> RKKIHQWYYRADDLEHKTALLVHLLKQPEATRSIVFVRKRERVHELANWLREAGINNCYLEGEMVQGKRNEAIKRLTEGRVNV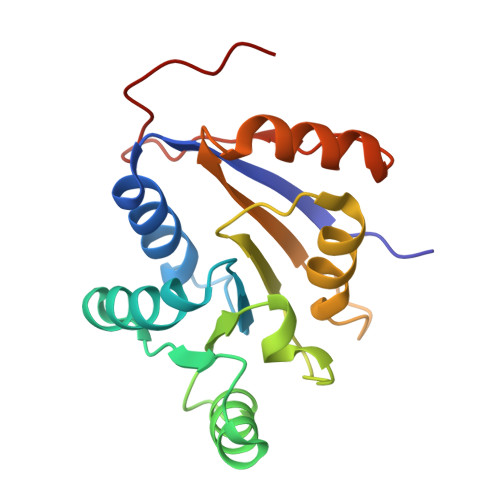LVATDVAARGIDIPDVSHVFNFDMPRSGDTYLHRIGRTARAGRKGTAISLVEAHDHLLLGKVGRYIEEPIKARVIDELRPKTRAPSE>[2x]SKKDLTMEDLT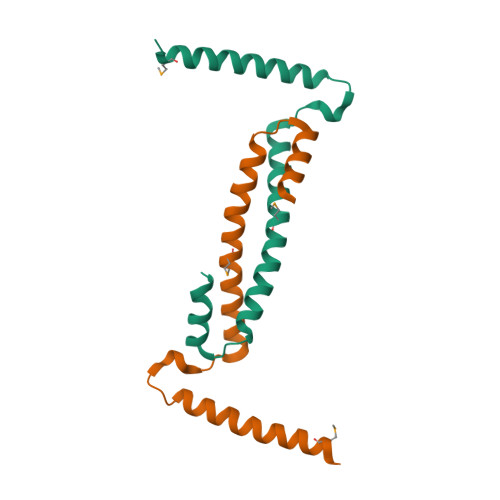AKISQLTVENRELRKALGSTADPRDRPLTATEKEAQLTATVGAMSAAAAKKIEARVRTIFSKVVTQKQVDDALKGLS>SGGGLPSTVIAISYFEGFVKLAAEWIVTEMPTTEIDGKTYTSGKLYIKMPETLDTDIKKSAMLFYKKQGLNETQMSTNHRNYPIHIVSKEEGDTLEVYDMPTILSGIDKAIDMYFRVGHIGKTTEQQLA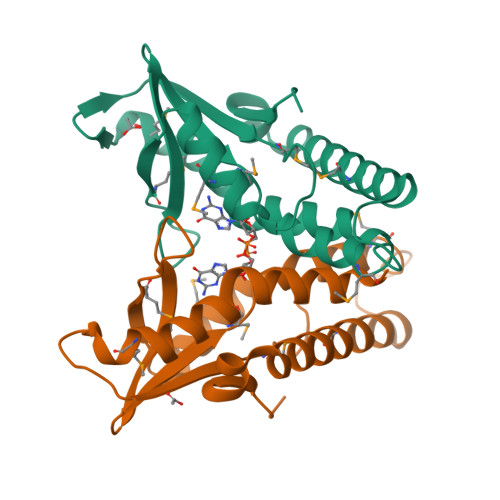EDNEMNNFKRVLQLLINEDSFCRECVEILRQA[2x]> STTTNSNSIGRPNLVALTRATTKLIYSDIVATQR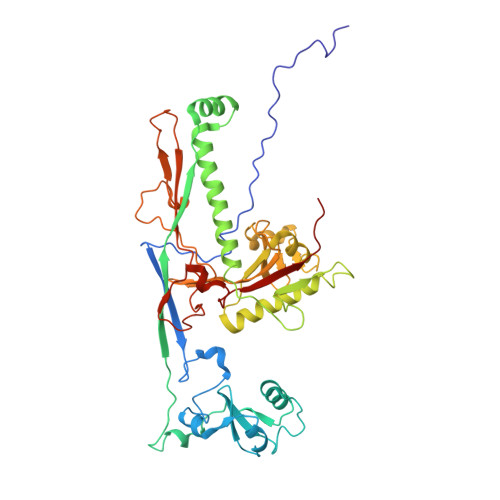TNQPVAAFYGIKYLNPDNEFTFKTGATYAGEAGYVDREQITELTEESKLTLNKGDLFKYNNIVYKVLEDTPFATIEESDLELALQIAIVLLKVRLFSDAASTSKFESSDSEIADARFQINKWQTAVKSRKLKTGITVELAQDLEANGFDAPNFLEDLLATEMADEINKDILQSLITVSKRYKVTGITDSGFIDLSYASAPEAGRSLYRMVCEMVSHIQKESTYTATFCVASARAAAILAASGWLKHKPEDDKYLSQNAYGFLANGLPLYCDTNSPLDYVIVGVVENIGEKEIVGSIFYAPYTEGLDLDDPEHVGAFKVVVDPESLQPSIGLLVRYALSANPYTVAKDEKEARIIDGGDMDKMAGRSDLSVLLGVKLPKIIIDE> MDNQCTVQVRLELGHRAQLRKKPTTEGFTHDWMVFVRGPEQCDIQHF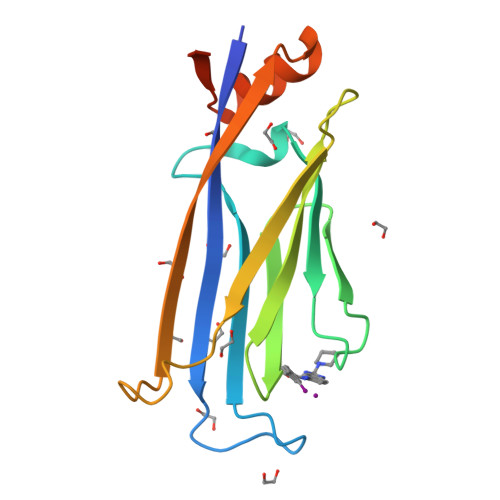VEKVVFWLHDSFPKPRRVCKEPPYKVEESGYAGFIMPIEVHFKNKEEPRKVCFTYDLFLNLEGNPPVNHLNHLRCEKLTFNNPTTEFRYKLLRAGGVMVMPEGAHHHHHH> GPLPKPTLWAEPGSVITQGSPVTLRCQGSLETQEYHLYREKKTALWITRIPQELVKKGQFPILSITWEHAGRYCCIYGSHTVGLSESSDPLELVVTG

LILRA3 is a soluble protein, the only secreted member of the LILR family, and contains four Ig-like domains (D1, D2, D3, and D4). As opposed to Group 2 LILRs, Group 1 members display high sequence similarity and are predicted to bind to HLA class I molecules (HLAIs). Further, LILRA3 is the only non-membrane-bound LILR, and its function was predicted to be antagonistic with HLA-binding Group 1 LILRs. Here, we report the binding properties of the LILRA3 D1 and D1D2 domains to HLAIs (classical HLA-A*0201 and non-classical HLA-G1) as analyzed by BIAcore® surface plasmon resonance (SPR) analysis, as well as the crystal structure of the LILRA3 D1 domain.

Based on the previous observation that the first two domains (D1 and D2) of Group 1 LILRs are responsible for binding to HLAIs and to determine if LILRA3 interacts with HLAIs, the first or first and second N-terminal domains of LILRA3 (D1, residues 1–97; and D1D2, residues 1–197, respectively) were expressed in Escherichia coli, followed by purification from inclusion bodies, and renaturation via dilution refolding method. The overall structure of the LILRA3 D1 domain has characteristics consistent with Ig-like domain structures and also displays properties unique to the LILR family. The structure is primarily composed of β strands arranged into two anti-parallel β sheets, with one β sheet containing three anti-parallel β strands (A, B and E) and the other containing four anti-parallel β strands (C, F, G and A′). Like the crystal structure of LILRB1 D1D2 and B2 D1D2, the D1 structure of LILRA3 also has a pocket-type hydrophobic core surrounded by the C and E strands and two 310 helices between the two strands. Most of the hydrophobic residues on the strands and the 310 helices face toward the interior of this hydrophobic core, which causes the hydrophilic residues on the adjacent loop region to protrude outside of the core. This hydrophobic core not only contains some important residues for direct binding to HLAIs but also pushes the adjacent hydrophilic residues (e.g., Tyr38, Glu40, Lys41, Lys42 and Glu68) to assume a proper conformation for its binding to HLAIs, unlike the residues of Group 2 members and LILRA2, where the two 310 helices between the C and E strands cannot be seen by helix-strand transitions. There is also a disulfide bond between cysteine residues 26 and 75, which clearly indicates that of the two neighboring cysteines (Cys74 and Cys75) in LILRA3 D1, Cys75 provides the correct conformation for native structure through its disulfide bond between the B and F strands. Some polar interactions may not exist in the LILRA3 D1/HLA-A*0201 complex because the amino acids at positions 36 and 76 were replaced with histidine and isoleucine from arginine (Arg36→His36) and tyrosine (Tyr76→Ile76). Again, the crystal structure of LILRA3 D1 displays that Lys42 forms a hydrogen bond with Glu68 of LILRA3 D1, rendering Lys42 unable to bind to Asp96 of the α3 domain of HLA-A*0201.> MENTENSVDSKSIKNLEPKIIHGSESMDSGISLDNSYKMDYPEMGLCIIINNKNFHKSTGMTSRSGTDVDAANLRETFRNLKYEVRNKNDLTREEIVELM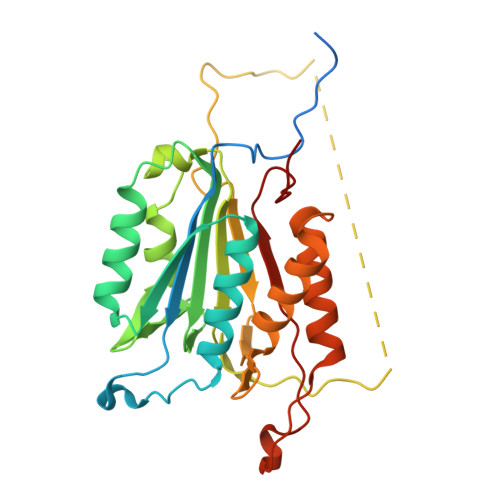RDVSKEDHSKRSSFVCVLLSHGEEGIIAGTNGPVDLKKITNFFRGDRCRSLTGKPKLFIIQACRGTELDCGIETDSGVDDDMACHKIPVEADFLYAYSTAPGYYSWRNSKDGSWFIQSLCAMLKQYADKLEFMHILTRVNRKVATEFESFSFDATFHAKKQIPCIHSMLTKELYFYHL>GNPPEIVRHIVFNRYKSQLSQ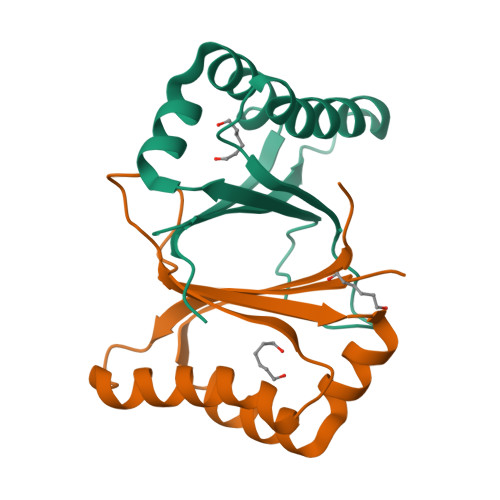KQIDQIIADYGNLQNIAPEMKEWKWGTDLGPAVEDRADGFTHAYESTFHSVADFLNFFYSPPALEFAKEFFPACEKIVVLNYIINE[12x]>[8x]GAMAPLTQDRIVVTALGILDAEGLDALSMRRLAQELKTGHASLYAHVGNRDELLDLVFDIVLTEVEVPEPEPGRWAEQVKEMCRSLRRMFLAHRDLARIAIDRVPLGPNGMVGMERTMNL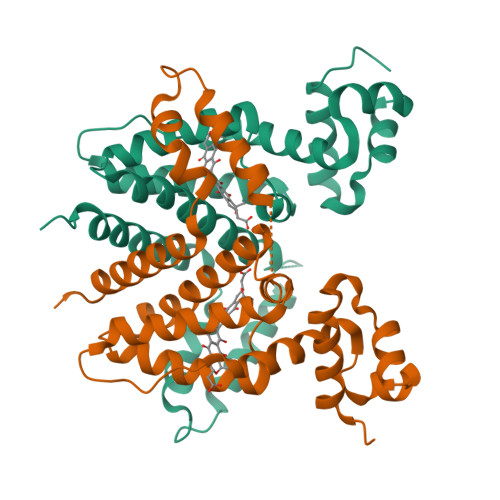LRSGGLHDELAAYGGDLLSTFVTAEALEQSSRNPGTEQGREQAGVFADQLHGYLKSLPATSFPNLVHLAGPITSLDSDRRFELGLEIIIAGLLAGAGEAADDQVRTAGSPPAES> QKQRAPRRRCQQPKMLS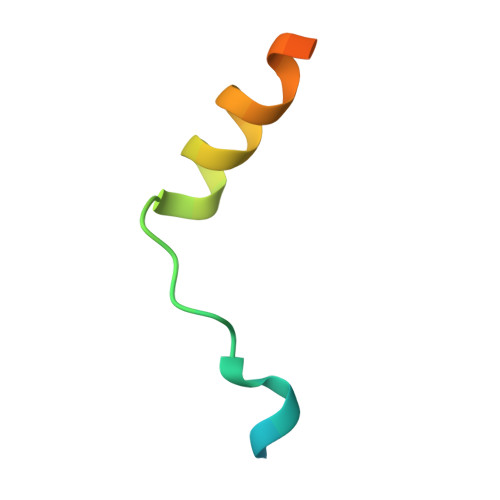SPEDTMYYNQLNGTLEYQG>[4x]MAGDSEQTLQNHQQPNGGE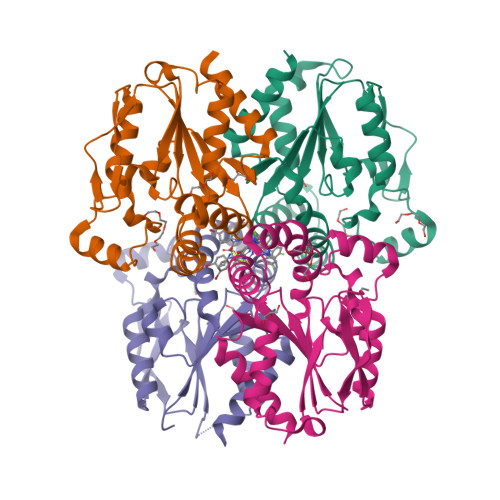PFLIGVSGGTASGKSSVCAKIVQLLGQNEVDYRQKQVVILSQDSFYRVLTSEQKAKALKGQFNFDHPDAFDNELILKTLKEITEGKTVQIPVYDFVSHSRKEETVTVYPADVVLFEGILAFYSQEVRDLFQMKLFVDTDADTRLSRRVLRDISERGRDLEQILSQYITFVKPAFEEFCLPTKKYADVIIPRGADNLVAINLIVQHIQDILNGGPSKRQTNGCLNGYTPSRK> MELKNSISDYTEAEFVQLLKEIEKENVAATDDVLYVLLEHFVKITEHPDGQDLIYYPSDNRDDSPEGIV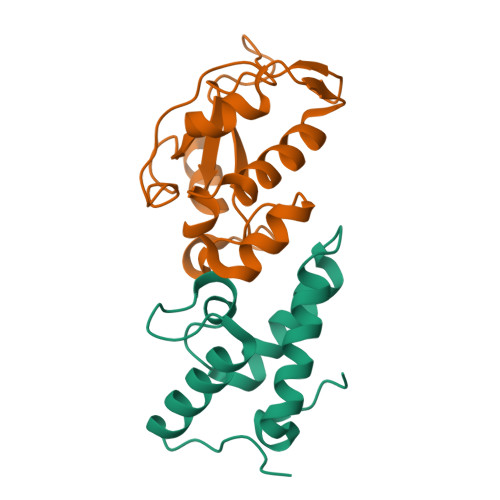KEIKEWRAANGKPGFKQG;> RNKPGKATGKGKPVNNKWLNNAGKDLGSPVPDRIANKLRDKEFKSFDDFRKKFWEEVSKDPELSKQFSRTQNDRMKVGRAPQTRTQDVSGKRQSFELHHEKPISQNGGVYDMDNISVVTPKRHIDIH> MGSSHHHHHHSSGENLYFQGSHMVGEKEYKAWEKKLRANEKELVKEYTANAKPFNTYLRANEGKLGFKPEIDKKILKLDEALKKSKLSETVQVYRGDDTSIFGKEFQNSIYQGNKVNRELFRKLRDEYQGKIRTEYGYLSTSIVSNQQFAMRPVLTTLKVPKGAHA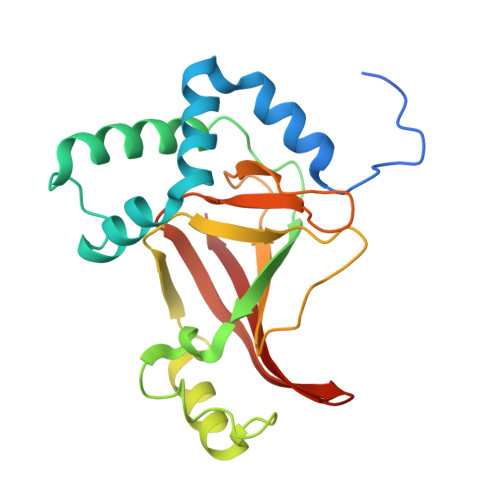GYVDKISQYKGQYELLLPRNTKYKIDKMYIIVNKGSETIKIEATVQP>[3x]MADPRPDPDELARRAAQVIADRTGIGEHDVAVVLGSGWLPAVAALGSPTTVLPQAELPGFVPPTAAGHAGELLSVPIGAHRVLVLAGRIHAYEGHDLRYVVHPVRAARAAGAQIMVLTNAAGGLRADLQVGQPVLISDHLNLTARSPLVGGEFVDLTDAYSPRLRELARQSDPQLAEG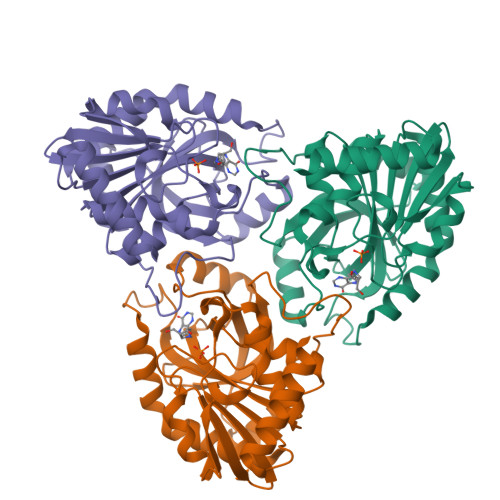VYAGLPGPHYETPAEIRMLQTLGADLVGMSTVHETIAARAAGAEVLGVSLVTNLAAGITGEPLSHAEVLAAGAASATRMGALLADVIARF The dipeptidyl peptidases (DPP) 8 and 9 are serine proteases of the dipeptidyl peptidase 4 activity/structure homologues (DASH) subfamily which cleave post-proline bonds two residues from the N-terminus of a substrate. While DPP4 and FAP are extracellular or secreted proteases, DPP8 and DPP9 are located intracellularly to the cytoplasm and nucleus. There, they play important roles in diverse biological processes such as pyroptosis or ubiquitin-mediated proteolysis, turning them into promising targets for chemical probe and anti-inflammatory or anticancer drug discovery. Here, we show the exploration of the natural product Sulphostin, a DPP4 inhibitor, as a starting point for DPP8/9 inhibitor development.

To elucidate the structural determinants underlying the formation of the reversible enzyme-inhibitor complex, we solved the X-ray structure of Sulphostin in complex with a catalytically dead DPP9 S730A mutant. In this experiment, a much larger electron density matching the complete structure of Sulphostin was found in the active site, confirming that the reversible enzyme-inhibitor complex is formed with a structurally intact Sulphostin residue and the (S)-3-aminopiperidin-2-one moiety is released only after nucleophilic attack by the active site serine. Sulphostin adopts a substrate-like binding mode, occupying both the S2 and S1 sub-sites with the aminopiperidine-2-one moiety, and with the amino group of the (S)-3-aminopiperidine-2-one forming a hydrogen-bonded ion pair to the glutamates E248 and E249 of the EE-helix. Of note, E248 and E249 line the end of the substrate binding tunnel and typically bind the N-terminus of substrate proteins. The (S)-3-aminopiperidine-2-one is thus not a “simple” proline mimic but structurally optimized to span two substrate binding sub-sites and to interact, in analogy to natural substrates, with substrate binding residues in the EE helix. Of note, the analysis of the structure also revealed an elaborate hydrogen bonding pattern between Sulphostin and DPP9, which matched the observed hydrogen bonds in the covalently conjugated wild-type DPP9 structure. After forming a non-covalent enzyme-inhibitor complex, the active site serine attacks the phosphotriamide moiety, most probably via a SN2(P) mechanism.

>[4x]MPAARFQVQKHSWDGLRSIIHGSRKYSGLIVNKAPHDFQFVQKTDESGPHSHRLYYLGMPYGSRENSLLYSEIPKKVRKEALLLLSWKQMLDHFQATPHHGVYSREEELLRERKRLGVFGITSYDFHSESGLFLFQASNSLFHCRDGGKNGFMVSPMKPLEIKTQCSGPRMDPKICPADPAFFSFINNSDLWVANIETGEERRLTFCHQGLSNVLDDPKSAGVATFVIQEEFDRFTGYWWCPTASWEGSEGLKTLRILYEEVDESEVEVIHVPSPALEERKTDSYRYPRTGSKNPKIALKLAEFQTDSQGKIVSTQEKELVQPFSSLFPKVEYIARAGWTRDGKYAWAMFLDRPQQWLQLVLLPPALFIPSTENEEQRLASARAVPRNVQPYVVYEEVTNVWINVHDIFYPFPQSEGEDELCFLRANECKTGFCHLYKVTAVLKSQGYDWSEPFSPGEDEFKCPIKEEIALTSGEWEVLARHGSKIWVNEETKLVYFQGTKDTPLEHHLYVVSYEAAGEIVRLTTPGFSHSCSMSQNFDMFVSHYSSVSTPPCVHVYKLSGPDDDPLHKQPRFWASMMEAASCPPDYVPPEIFHFHTRSDVRLYGMIYKPHALQPGKKHPTVLFVYGGPQVQLVNNSFKGIKYLRLNTLASLGYAVVVIDGRGSCQRGLRFEGALKNQMGQVEIEDQVEGLQFVAEKYGFIDLSRVAIHGWAYGGFLSLMGLIHKPQVFKVAIAGAPVTVWMAYDTGYTERYMDVPENNQHGYEAGSVALHVEKLPNEPNRLLILHGFLDENVHFFHTNFLVSQLIRAGKPYQLQIYPNERHSIRCPESGEHYEVTLLHFLQEYLHHHHHH>SNAMKLTPNFYRDRVCLNVLAGSKDNAREIYDAAEGHVLVGVLSKNYPDVASAVVDMRDYAKLIDNALSVGLGAGDPNQSAMVSEISRQVQPQHVNQVFTGVATSRALLGQNETVVNGLVSPTGTPGMVKISTGPLSSGAADGIVPLETAIALLKDMGGSSIKYFPMGGLKHRAEFEAVAKACAAHDFWLEPTGGIDLENYSEILKIALDAGVSKIIPHIYSSIIDKASG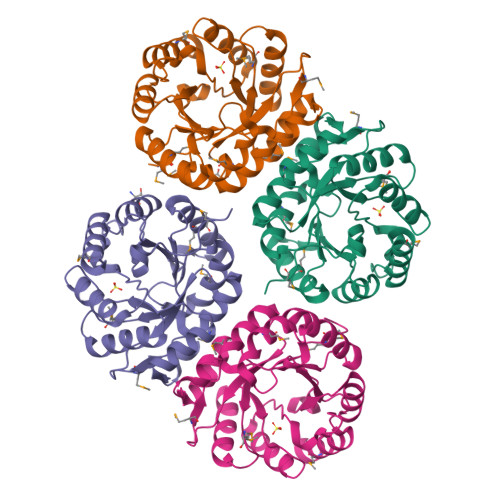NTRPADVRQLLEMTKQLVK[4x]>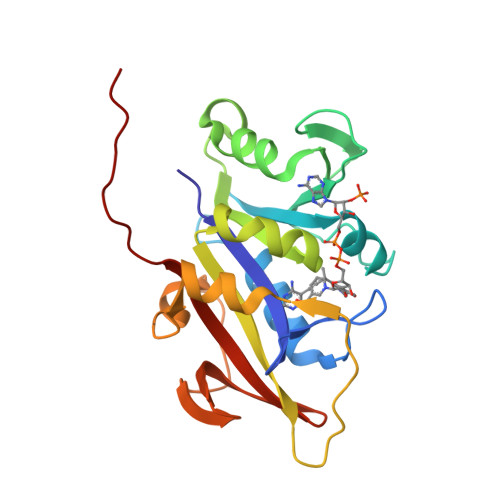[2x]KVPVVGIVAALLPEMGIGFQGNLPWRLAKEMKYFREVTTLTNDNSKQNVVIMGRKTWESIPQKFRPLPKRINVVVSRSFDGELRKVEDGIYHSNSLRNCLTALQSSLANENKIERIYIIGGGEIYRQSMDLADHWLITKIMPLPETTIPQMDTFLQKQELEQRFYDNSDKLVDFLPSSIQLEGRLTSQEWNGELVKGLPVQEKGYQFYFTLYTKKLEHHHHHHHH> GSHMSNQALYEK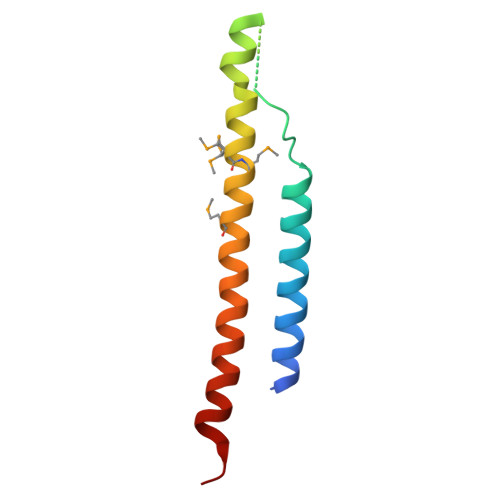LEQTRTILSVKLAELINITTIADRNDDDEGSFAQENSELAVATTSVMMVNNQTMQLIKNVQDLLILTRSIKEKWLLNQIP>[4x]GMTSFDRPFEAARPDGENPSAHETLAEGGRLRPEATYTIPARQGRAIRMAQGEALMVINRDGSQIG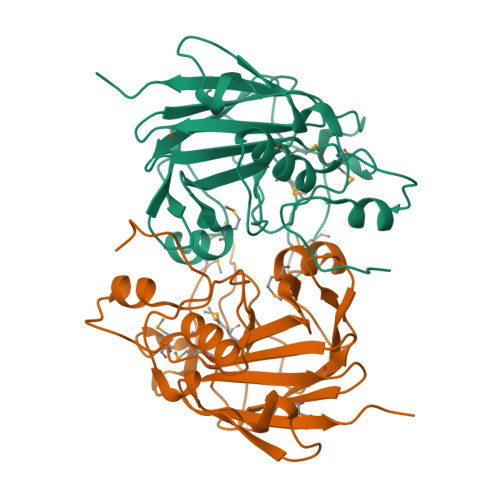DFWAFVEGDCGEYLSMEHLRPTLRRVSPRPGDVLVSNRRRPILTLLEDSSPGVHDTLVASCDVHRYAQLGHEGYHDNCTDNLRMALGALGLRPTTVPCPLNLWMNTPVVEGGAMEWRPPVSRRGDHVLFRAELDVVVVISCCPMDLLPINGEEAQPRALDVRLRPRPA> MSYYHHHHHHLESTSLYKKAGSHMDKEGFLNKVREAVDVVKLHIELGHTIRIISHRDADGITSAAILAKALGREGASFHISIVKQVSEDLLRELKDEDYKIFIFSDLGSGSLSLIKEYLKEKTVIILDHHPPENVKLEEKHILVNPVQFGANSVRDLSGSGVTYFFARELNEKNRDLAYIAIVGAVGDMQENDGVFHGMNLDIIEDGKSLGILEVKKELRLFGRETRPLYQMLAYATNPEIPEVTGDERKAIEWLKNKGFNPEKKYWELSEEEKKKLHDFLIIHMIKHGAGKEDIDRLIGDVVISPLYPEGDPRHEAREFATLLNATGRLNLGNLGVAVCLGDEEAFRKALKMVEDYKREQIEARKWLLQNWNSEVWEGDHVYVLYVGKSIRDTLVGIAASMAINAGLADPEKPVIVFADTDEDPN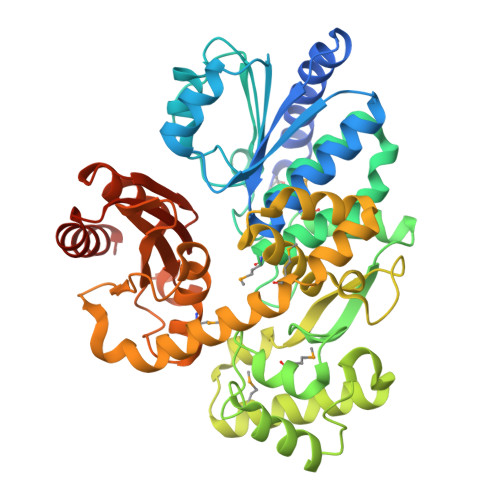LLKGSARTTERALAKGYNLGEALRKAAELVNGEGGGHAIAAGIRIPRARLAEFRKLIDKILGEQVSKGGDKSES> MLRLSSWNLKSQHHNVLRRSRPHIHKYRELNRWQRQAQGISKWDQSHSHRPLPYVERFNPESVGLTRGTSAFAWKWWHTQYPWLPNVPPEAAQIDEAQKQERRSHRPPAWDDEFAK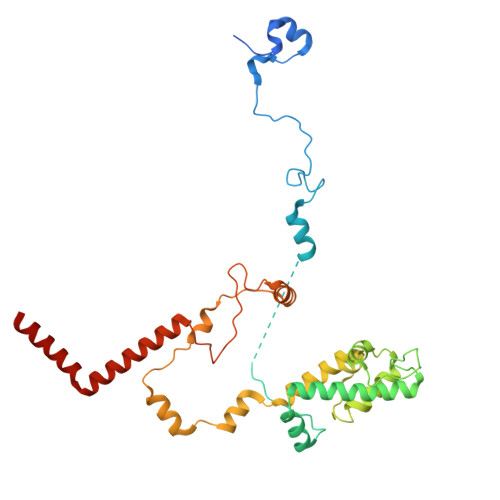VVLNMNDAEIREYLMSKLTDVIFLETQRDGYELRRLDFEGKPLTSLPEPRIIENFVLEEETIRERVIYQVVEGVFRLSPTSADRRELRSVANIIDYVLTHVRAARPTDRERRQERPITSAALAVMQKCPIQPQLGFVHALPHDTRDALLQEWERMHHLDWQFGKAVYTPRSKENVRGNLTWLREDRHYDQRMKFMQEVESGEARAKHMKLIAEAAGN> GAMGSPVSVQQSLAAYNQRKADLVNRSIAQMREATTLANGVLASLNLPAAIEDVSGDTVPQSILTKSRSVIEQGGIQTVDQLIKELPELLQRNREILDESLRLLDEEEATDNDLRAKFKERWQRTPSNELYKPLRAEGTNFRTVLDKAVQADGQVKECYQSHRDTIVLLCKPEPELNAAIPSANPAKTMQGSEVVSVLKSLLSNLDEVKKEREGLENDLKSVNFDMTSKFLTALAQDGVINEEALSVTELDRVYGGLTTKVQESLKKQEGLLKNIQVSHQEFSKM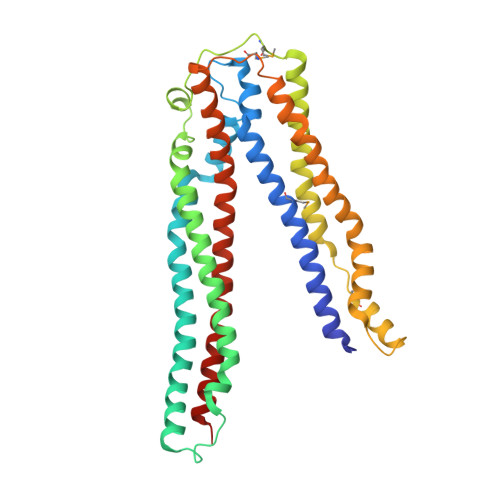KQSNNEANLREEVLKNLATAYDNFVELVANLKEGTKFYNELTEILVRFQNKCSDIVFARKTER>[2x]FQ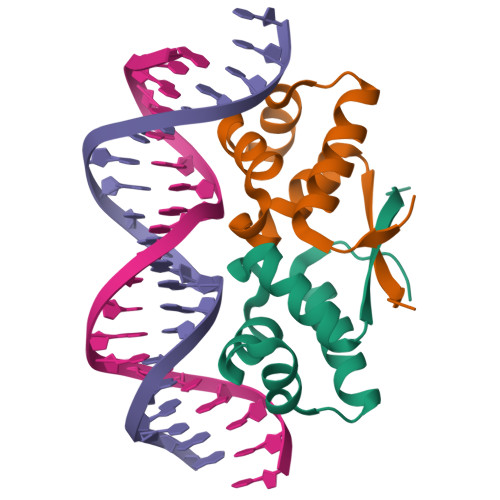KIYSPTQLANAMKLVRQQNGWTQSELAKKIGIKQATISNFENNPDNTTLTTFFKILQSLELSMTLCDAK>XFFYK[70x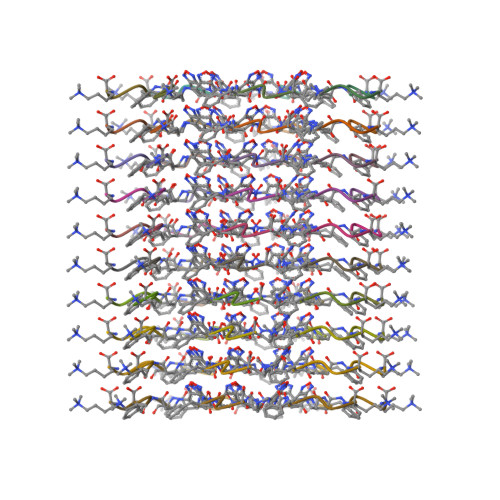]> GRTTRDDLINGNSASCADVIFIYARGSTETGNLGTLGPSIASNLESAFGKDGVWIQGVGGAYRATLGDNALPRGTSSAAIREMLGLFQQANTKCPDAT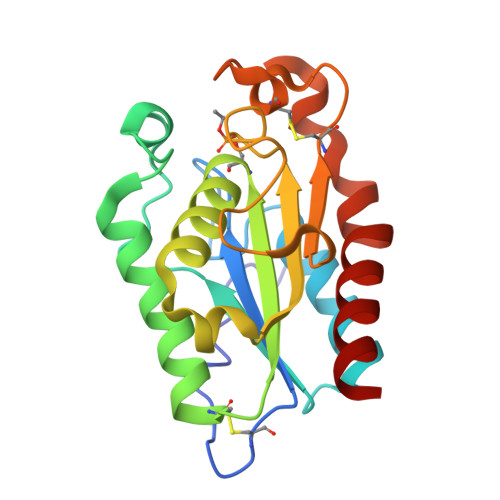LIAGGYXQGAALAAASIEDLDSAIRDKIAGTVLFGYTKNLQNRGRIPNYPADRTKVFCNTGDLVCTGSLIVAAPHLAYGPDARGPAPEFLIEKVRAVRG> GHMKQIAFIGLGHMGAPMATNLLKAGYLLNVFDLVQSAVDGLVAAGASAARSARDAVQGADVVISMLPASQHVEGLYLDDDGLLAHIAPGTLVLECSTIAPTSARKIHAAARERGLAMLDAPVSGGTAGAAAGTLTFMVGGDAEALEKARPLFEAMGRNIFH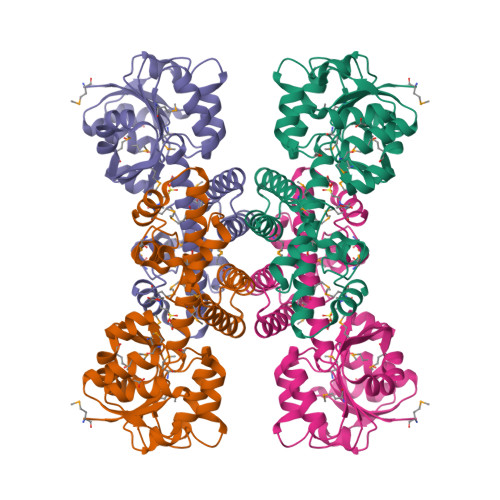AGPDGAGQVAKVCNNQLLAVLMIGTAEAMALGVANGLEAKVLAEIMRRSSGGNWALEVYNPWPGVMENAPASRDYSGGFMAQLMAKDLGLAQEAAQASASSTPMGSLALSLYRLLLKQGYAERDFSVVQKLFDPTQGQ3-[N-[BENZYLOXYCARBONYL]-PHENYLALANINYL-AMINO]-5-PHENYL-PENTANE-1-SULFONYLMETHYLBENZENE | C35 H38 N2 O5 S | 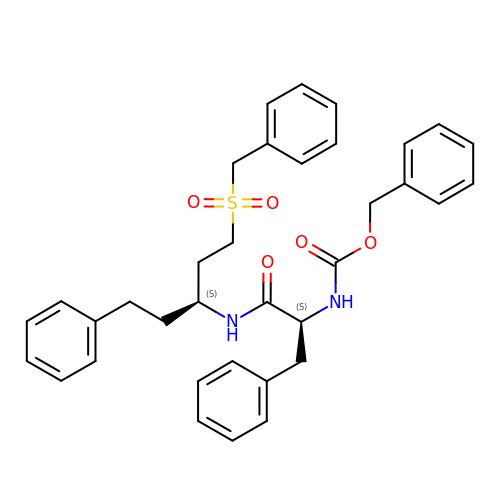VXIINIMESJGNGI-LQJZCPKCSA-N>MHHHHHHHHSSGLVPRGSAMGSKPLRIGVPNRVSYTDYVSKDKNPPGVRGYCIDVFEAAIELLPYPVPRTYILYGDGKRNPSYDNLVNEVVADNFDVAVGDITIVTNRTRYVDFTQPFIESGLVVVAPVKEAGTIEGIDSLVTSN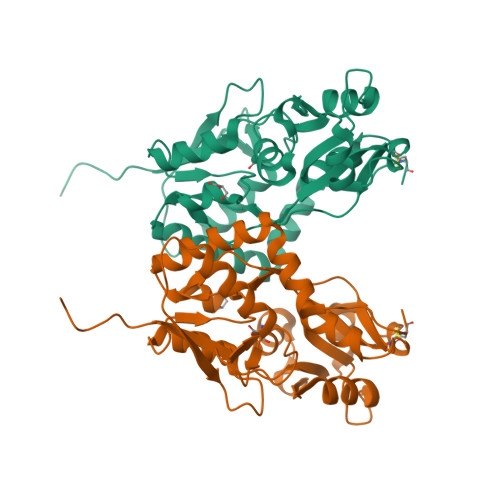EPIGVQDGTFARNYLINELNILPSRIVPLKDEEQYLSALQRGPNAGGVAAIVDELPYIEVLLTNSNCKFRTVGQEFTRTGWGFAFQRDSPLAVDMSTAILQLSEEGELEKIHRKWLNYKHECS[3x]N-(2,2-diphenylethyl)-1,5-dimethyl-N-[2-(methylamino)-2-oxidanylidene-ethyl]-6-oxidanylidene-pyridine-3-carboxamide | C25 H27 N3 O3 | 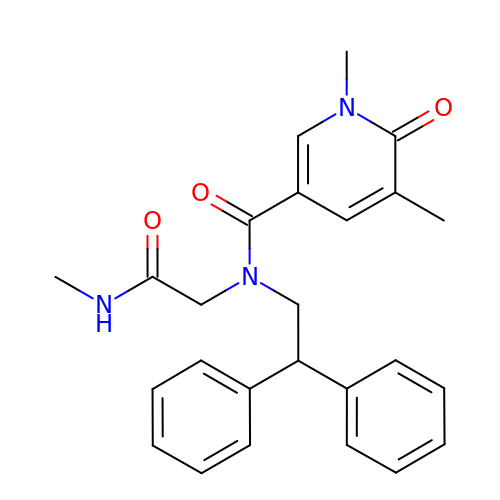YSBWPORVNMMWTB-UHFFFAOYSA-N> AFNNNPSSVGAYSSGTYRNLAQEMGKTNIQQKVNSTFDNMFGYNN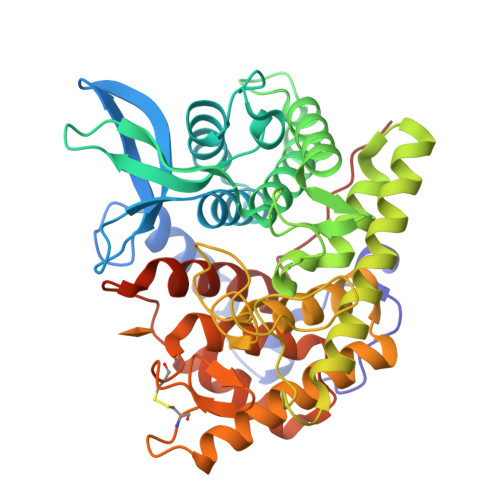TQQLYYPYTENGVYKAHYIKAINPDEGDDIRTEGQSWGMTAAVMLNKQEEFDNLWRFAKAYQKNPDNHPDAKKQGVYAWKLKLNQNGFVYKVDEGPAPDGEEYFAFALLNASARWGNSGEFNYYNDAITMLNTIKNKLMENQIIRFSPYIDNLTDPSYHIPAFYDYFANNVTNQADKNYWRQVATKSRTLLKNHFTKVSGSPHWNLPTFLSRLDGSPVIGYIFNGQANPGQWYEFDAWRVIMNVGLDAHLMGAQAWHKSAVNKALGFLSYAKTNNSKNCYEQVYSYGGAQNRGCAGEGQKAANAVALLASTNAGQANEFFNEFWSLSQPTGDYRYYNGSLYMLAMLHVSGNFKFYNNTFN>[4x]TPTDKHGGSDTRCPLMVKILDAVKGTPAGSV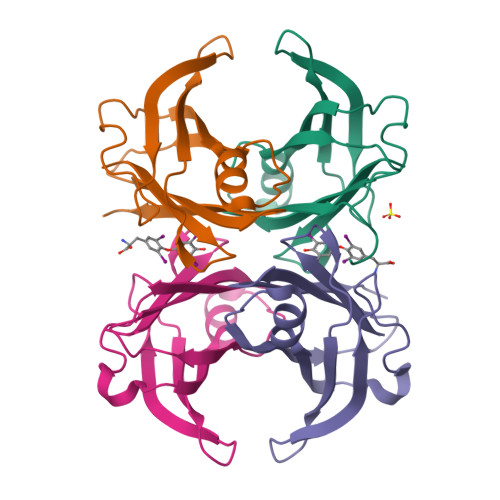ALKVSQKTADGGWTQIATGVTDATGEIHNLITEQQFPAGVYRVEFDTKAYWTNQGSTPFHEVAEVVFDAHPEGHRHYTLALLLSPFSYTTTAVVSSVHE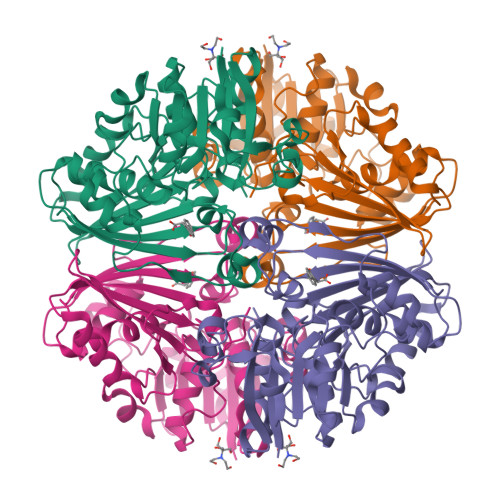>[2x]GSMQNRQVANATKVAVAGASGYAGGEILRLLLGHPAYADGRLRIGALTAATSAGSTLGEHHPHLTPLAHRVVEPTEAAVLGGHDAVFLALPHGHSAVLAQQLSPETLIIDCGADFRLTDAAVWERFYGSSHAGSWPYGLPELPGARDQLRGTRRIAVPGCYPTAALLALFPALAADLIEPAVTVVAVSGTSGAGRAATTDLLGAEVIGSARAYNIAGVHRHTPEIAQGLRAVTDRDVSVSFTPVLIPASRGILATCTARTRSPLSQLRAAYEKAYHAEPFIYLMPEGQLPRTGAVIGSNAAHIAVAVDEDAQTFVAIAAIDNLVKGTAGAAVQSMNLALGWPETDGLSVVGVAP>SNAMGEAATKSDRQQNQTRLWLNILRLHGLVFGDLNRQLLDETGLSLAKFDAMAQLARNPDGLSMGKLSGALKVTNGN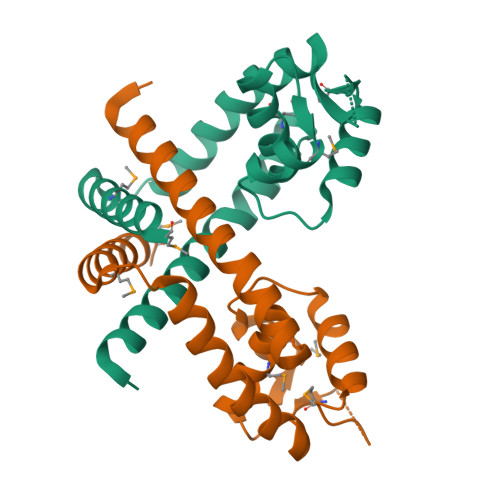VSGLVNRLIKDGMVVKAMSADDRRSFSAKLTDAGLTTFKQASEAHNRILAELLRAVSDQDMVEASAALRGILESMQTGASLD[2x]>MMEQVCDVFDIYAICACCKVESKNEGKKNEVFNNYTFRGLGNKGVLPWKCISLDMKYFRAVTTYVNESKYEKLKYKRCKYLNKETVDNVNDMPNSKKLQNVVVMGRTNWESIPKKFKPLSNRINVILSRTLKKEDFDEDVYIINKVEDLIVLLGKLNYYKCFILGGSVVYQEFLEKKLIKKIYFTRINSTYECDVFFPEINENEYQIISVSDVYTSNNTTLDFIIYKKTNNKMLNEQNCIKGEEKNNDMPLKNDDKDTCHMKKLTEFYKNVDKYKINYEN[2x];>DDDDEEEDDFVYFNFNKEKEEKNKNSIHPNDFQIYNSLKYKYHPEYQYLNIIYDIMMNGNKQSDRTGVGVLSKFGYIMKFDLSQYFPLLTTKKLFLRGIIEELLWFIRGETNGNTLLNKNVRIWEANGTREFLDNRKLFHREVNDLGPIYGFQWRHFGAEYTNMYDNYENKGVDQLKNIINLIKNDPTSRRILLCAWNVKDLDQMALPPCHILCQFYVFDGKLSCIMYQRSCDLGLGVPFNIASYSIFTHMIAQVCNLQPAQFIHVLGNAHV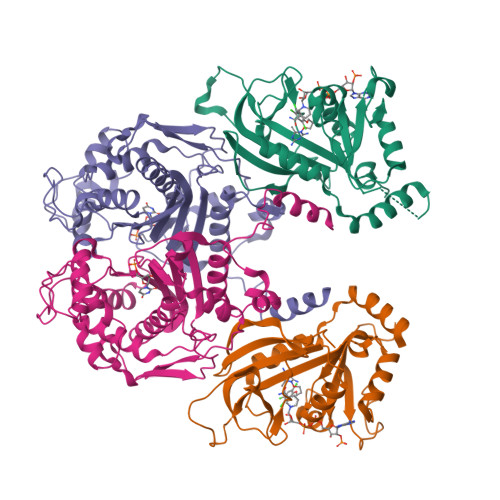YNNHIDSLKIQLNRIPYPFPTLKLNPDIKNIEDFTISDFTIQNYVHHEKISMDMAA[2x]>[4x]MPREYEFAEKILFTEEEIRTRIKEVAKRIADDYKGKGLRPYVNPLVLISVLKGSF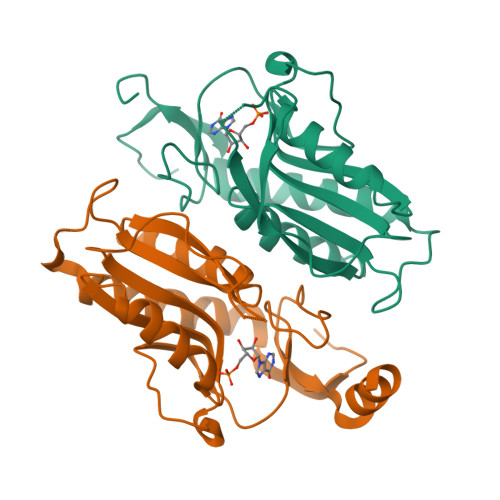MFTADLCRALCDFNVPVRMEFICVSSYGEGLTSSGQVRMLLDTRHSIEGHHVLIVEDIVDTALTLNYLYHMYFTRRPASLKTVVLLDKREGRRVPFSADYVVANIPNAFVIGYGLDYDDTYRELRDIVVLRPEVYAEREAARQKKQRAIGSADTDRDAKREFHSKY>GPQRTCGSELNMEQIRRTEPLKYQRITDWENQIKLHSRSVPSSTILIPVVVHVVYNNSAQNISDAQIISQIQVLNEDFRRMNADQANTPSAFANLAGNANIEFKLARRDPNGNTTNGITRTSTSTETFSMEMDNVKFSNLGGNNAWNTRRYLNIWVCNLGDDLLGYAQFPFEFQTKPNTDGVVIHYKHFGRDGSAESPYDKGRTATHAVGHWLDLRHIWGDDGGSCSGTDNIADTPNQGGY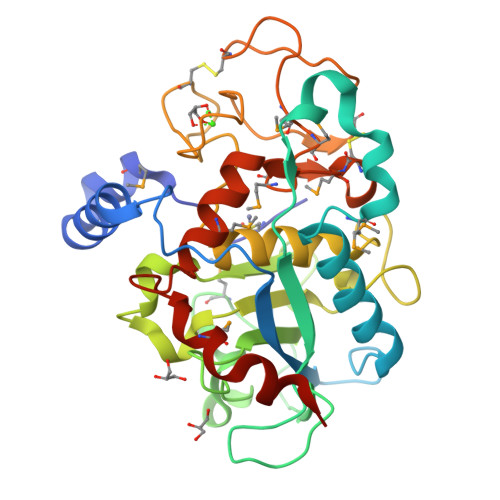NEGCPSFPKTDHCTNTSPGVMFMNYMDYTYDACMNLFTKGQVERMRSLFDTQTGIRREMQIYANELTNPLSFS[2x]> MKGGFTGGDEYQKHFLPRDYLATYYSFDGSPSPEAEMLKFNLECLHKTFGPGGLQG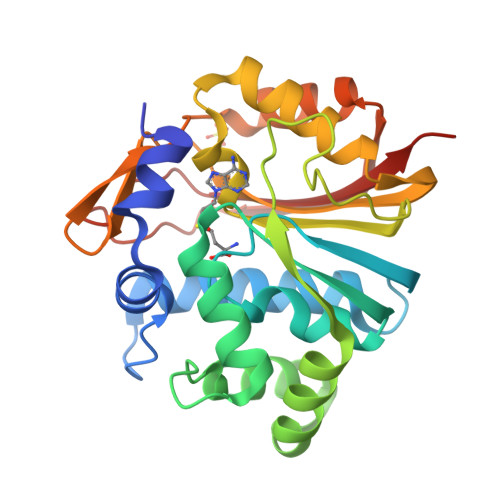DTLIDIGSGPTIYQVLAACDSFQDITLSDFTDRNREELEKWLKKEPGAYDWTPAVKFACELEGNSGRWEEKEEKLRAAVKRVLKCDVHLGNPLAPAVLPLADCVLTLLAMECACCSLDAYRAALCNLASLLKPGGHLVTTVTLRLPSYMVGKREFSCVALEKGEVEQAVLDAGFDIEQLLHSPQSYSVTNAANNGVCCIVARKKPGP>SNAMSQFMNLEGKVALVTGASRGIGKAIAELLAERGAKVIGTATSESGAQAISDYLGDNGKGMALNVTNPESIEAVLKAITDEFGGVDILVNNAGITRDNLLMRMKEEEWSDIMETNLTSIFRLSKAVLRGMMKKRQGRIINVGSVVGTMGNAGQ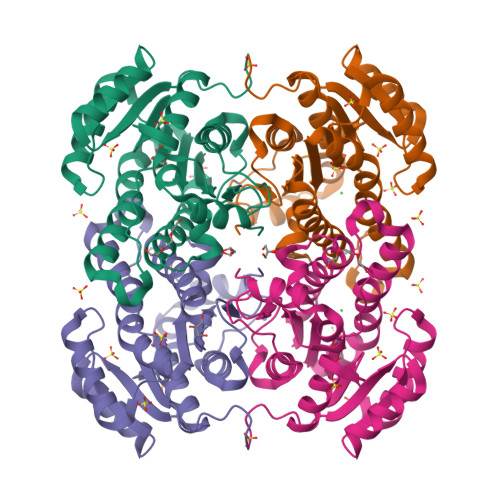ANYAAAKAGVIGFTKSMAREVASRGVTVNTVAPGFIETDMTKALNDEQRTATLAQVPAGRLGDPREIASAVAFLASPEAAYITGETLHVNGGMYMI[2x]>[8x]MKSVVTTVIAAADAAGRFPSSSDLESVQGSIQRAAARLEAAEKLAGNIDAVATEAYNACIKKYPYLNNAGEANSTDTFKAKCARDIKHYLRLIQYCLVVGGTGPLDEWGIAGQREVYRALGLPTAPYVEALSFARNRGCAPRDMSAQALTEYNALLDYAINSLS;>[8x]MLDAFSRAVVSADASTSTVSDIAALRAFVASGNRRLDAV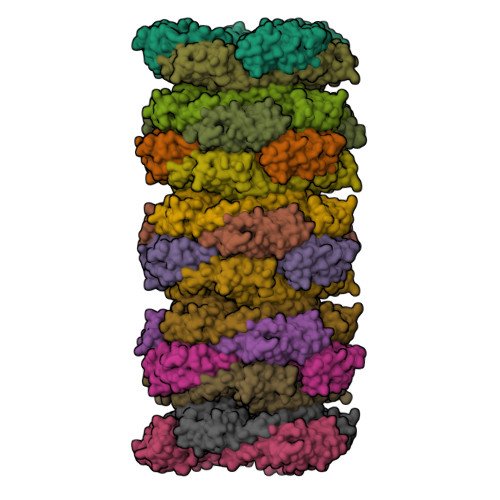NAIASNASCMVSDAVAGMICENQGLIQAGGNCYPNRRMAACLRDAEIILRYVTYALLAGDASVLDDRCLNGLKETYAALGVPTTSTVRAVQIMKAQAAAHIQDTPSEARAGAKLRKMGSPVVEDRCASLVAEASSYFDRVISALS>MHHHHHHHGAAMKSYFVTMGFNETFLLRLLNETSAQKEDSLVIVVPSPIVSGTRAAIESLRAQISRLNYPPPRIYEIEITDFNLALSKILDIILTLPEPIISDLTMGMRMINTLILLGIIVSRKRFTVYVRDEGGGSRVISFNDNTIRALMRDYSREEMKLLNVLYETKG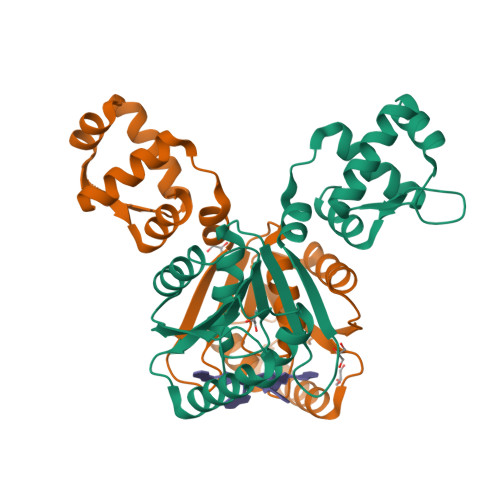TGITELAKMLDKSEKTLINKIAELKKFGILTQKGKDRKVELNELGLNVIKLNKSVIESSKSSEELVKENKGKEVNIPY[2x]>MDNSHDSDSVFLYHIPCDNCGSSDGNSLFSDGHTFCYVCEKWTAGNEDTKERASKRKPSGGKPMTYNVWNFGESNGRYSALTARGISKETCQKAGYWIAKVDGVMYQVADYRDQNGNIVSQKVRDKDKNFKTTGSHKSDALFGKHLWNGGKKIVVTEGEIDMLTVMELQDCKYPVVSLGHGASAAKKTCAANY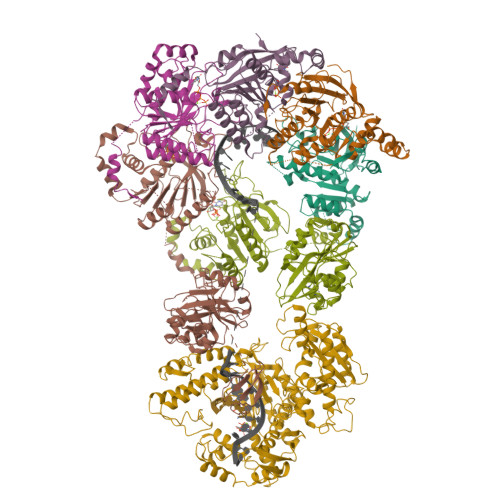EYFDQFEQIILMFDMDEAGRKAVEEAAQVLPAGKVRVAVLPCKDANECHLNGHDREIMEQVWNAGPWIPDGVVSALSLRERIREHLSSEESVGLLFSGCTGINDKTLGARGGEVIMVTSGSGMGKSTFVRQQALQWGTAMGKKVGLAMLQESVEETAEDLIGLHNRVRLRQSDSLKREIIENGKFDQWFDELFGNDTFHLYDSFAEAETDRLLAKLAYMRSGLGCDVIILDHISIVVSASGESDERKMIDNLMTKLKGFAKSTGVVLVVICHLKNPDKGKAHEEGRPVSITDLRGSGALRQLSDTIIALERNQQGDMPNLVLVRILKCRFTGDTGIAGYMEYNKETGWLEPSSYSGEEESHSESTDWSNDTDF[6x];> MIVSAIAANALLESVTKFHCGVIYDYSTAEYVSYRPSDFGAYLDALEAEVARGGLIVFHNGHKYDVPALTKLAKLQLNREFHLPRENCIDTLVLSRLIHSNLKDTDMGLLRSGKLPGKRFGSHALEAWGYRLGEMKGEYKDDFKRMLEEQGEEYVDGMEWWNFNEEMMDYNVQDVVVTKALLEKLLSDKHYFPPEIDFTDVGYTTFWSESLEAVDIEHRAAWLLAKQERNGFPFDTKAIEELYVELAARRSELLRKLTETFGSWYQPKGGTEMFCHPRTGKPLPKYPRIKTPKVGGIFKKPKNKAQREGREPCELDTREYVAGAPYTPVEHVVFNPSSRDHIQKKLQEAGWVPTKYTDKGAPVVDDEVLEGVRVDDPEKQAAIDLIKEYLMIQKRIGQSAEGDKAWLRYVAEDGKIHGSVNPNGAVTGRATHAFPNLAQIPGVRSPYGEQCRAAFGAEHHLDGITGKPWVQAGIDASGLELRCLAHFMARFDNGEYAHEILNGDIHTKNQIAAELPTRDNAKTFIYGFLYGAGDEKIGQIVGAGKERGKELKKKFLENTPAIAALRESIQQTLVESSQWVAGEQQVKWKRRWIKGLDGRKVHVRSPHAALNTLLQSAGALICKLWIIKTEEMLVEKGLKHGWDGDFAYMAWVHDEIQVGCRTEEIAQVVIETAQEAMRWVGDHWNFRCLLDTEGKMGPNWAICH> MASESSIPLYDCLIIGGGIAGLSSALSLVRTLHTAVVFDEGIHRNDQAPHLATVPTWDSQDPKRFRDAAKLNILSKYSTVEFANVKLEKVNQLTDGPYKGYFCVWDTKQRQWLGRKVILAMGVEDLLPTIDGFAECWTKGI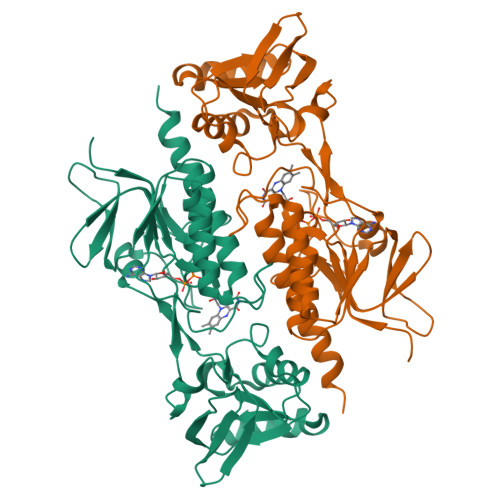FHCLVHRGYEERGSASGGVLAIDGDATFFAARHLAFQARNLTDHVVIYTHGNDELAQEVESQLGPCGFRAESRRIEKLVQHPERAQMEVHFEDGQSETVGFIVHRPRTSIRGPFAEQLGVEMTPEGHIKTQFPFNETTVSGVFVAGDAGSQFKIGTQAVVMGAFAAGGVQMQVNAEKWSQPLNSVVSQGHHHHHH> MEIKETYDFSSIVDLWNKNIGTVYPMNLELFKQNYINDRQRKKIMGAFNGEILIGFVIYKQWTYKSGSLKPNHKIGYINSIIVDINFRHQGIGTKLLDAAEEELINSGVKILR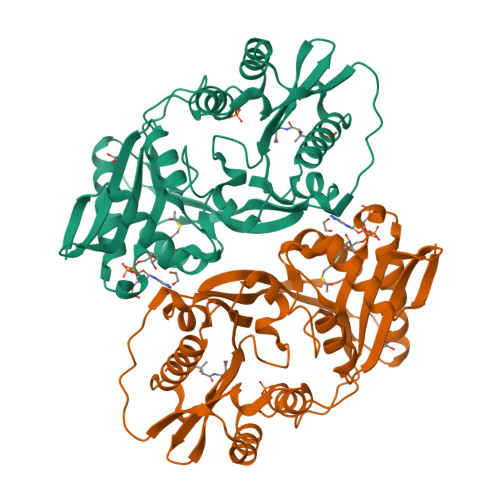CGSDTYHFFPGIPLECLPSEEFFLVRGYKMQDYFYDLIGDVSKVDFKKPSIKDGFKVNVMKPEDRKGLFEFLEKSFSGRWLEEFIEFFQVGMKERDIVLIKYKTSVIGFSHIYDNKSSFIGPPIYWKALLGHNYGGLGPIGIDKTYRKQGLGRLLLYESLQILKKREVKKMVIDWTEKDIINFYGRFNFMPWKAYRKATKEVKDGKGGGHHHHHH> GAQVSTQ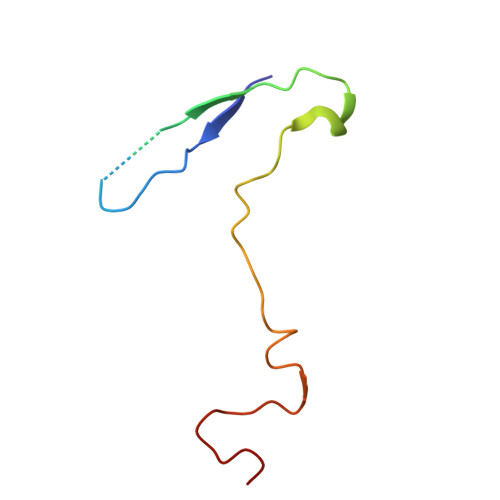KTGAHETSLSASGNSIHYTNINYYKDAASNSANRQDFTQDPGKFTEPVKDIMVKSLPALN> PQAKYRHDYRAPDYQITDIDLTFDLDAQKTVVTAVSQAVRHGASDAPLRLNGEDLKLVSVHINDEPWTAWKEEEGALVISNLPERFTLKIINEISPAANTALEGLYQSGDALCTQCEAEGFRHITYYLDRPDVLARFTTKIIADKIKYPFLLSNGNRVAQGELENGRHWVQWQDPFPKPCYLFALVAGDFDVLRDTFTTRSGREVALELYVDRGNLDRAPWAMTSLKNSMKWDEERFGLEYDLDIYMIVAVDFFNAGAMENKGLNIFNSKYVLARTDTATDKDYLDIERVIGHEYFHNWTGNRVTCRDWFQLSLKEGLTVFRDQEFSSDLGSRAVNRINNVRTMRGLQFAEDASPMAHPIRPDMVIEMNNFYTLTVYEKGAEVIRMIHTLLGEENFQKGMQLYFERHDGSAATCDDFVQAMEDASNVDLSHFRRWYSQSGTPIVTVKDDYNPETEQYTLTISQRTPATPDQAEKQPLHIPFAIELYDNEGKVIPLQKGGHPVNSVLNVTQAEQTFVFDNVYFQPVPALLCEFSAPVKLEYKWSDQQLTFLMRHARNDFSRWDAAQSLLATYIKLNVARHQQGQPLSLPVHVADAFRAVLLDEKIDPALAAEILTLPSVNEMAELFDIIDPIAIAEVREALTRTLATELADELLAIYNANYQSEYRVEHEDIAKRTLRNACLRFLAFGETHLADVLVSKQFHEANNMTDALAALSAAVAAQLPCRDALMQEYDDKWHQNGLVMDKWFILQATSPAANVLETVRGLLQHRSFTMSNPNRIRSLIGAFAGSNPAAFHAEDGSGYLFLVEMLTDLN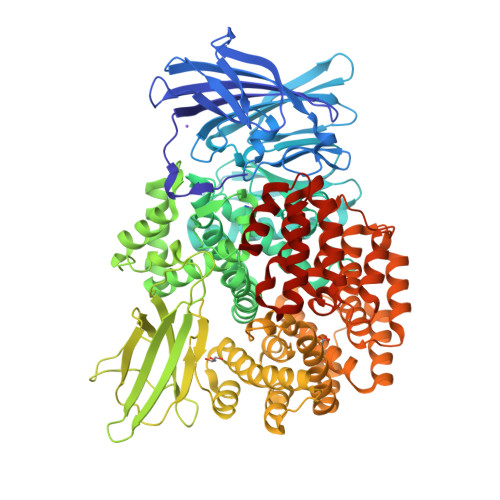SRNPQVASRLIEPLIRLKRYDAKRQEKMRAALEQLKGLENLSGDLYEKITKALA> MADSREKVTLGTVVDCFKGKAVSSKVVPGDVGLINLSDMGTLGIQYHQLRTFQMDRRQLLRYLLEDGDVLIASKGTLKKVCVFHKQNRDVVASSNITVLRPQKLLRGYYIKFFLDSPIGQALLDAADHGKDVINLSTKELLDIPIPVIPLVKQDYLINHYLRGLTDYHRKLNRAE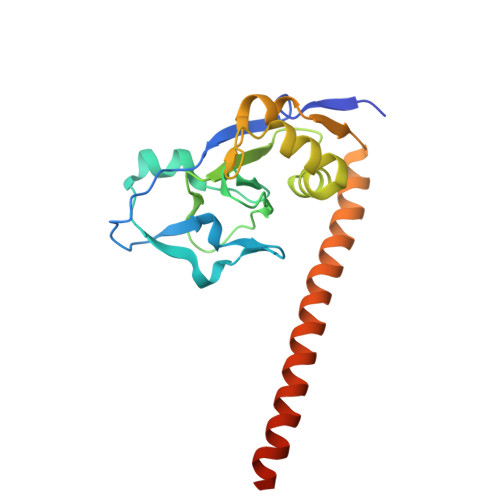QEWEYIQNEIQKGLGLEHHHHHH>GSHMDSTTIQQNKDTLSQIVVFPTGNYDKNEANAMVNRLANIDGKYLNALKQNNLKIKLLSGKLTDEKEYAYLKGVVPRGWEGTGKTWDDVPGLGGSTVALRIGFSNKGKGHDAINLELHETAHAIDHIVLNDISKSAQFKQIFAKEGRSLGNVNYLGVYPEEFFAESF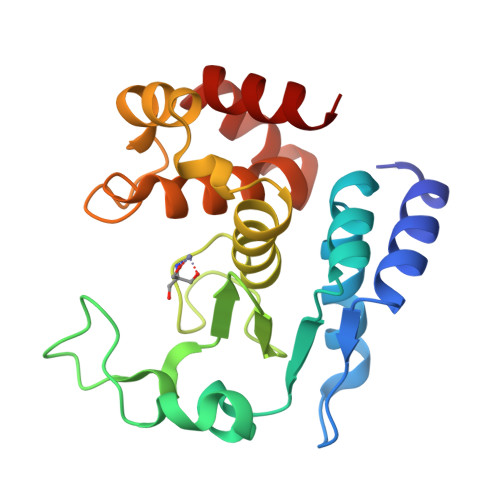AYYYLNQDTNSKLKSACPQTYSFLQNLAK[2x]>[4x]AHI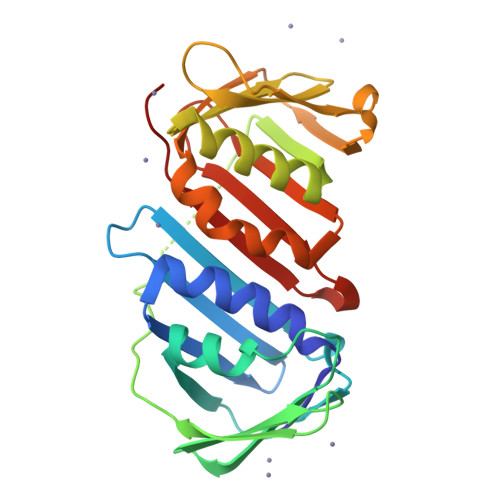VYDDVRDLKAIIQALLKLVDEALFDIKPEGIQLVAIDKAHISLIKIELPKEMFKEYDVPEEFKFGFNTQYMSKLLKAAKRKEEIIIDADSPEVVKLTLSGALNRVFNVNNIEVLPPEVPEVNLEFDIKATINASGLKNAIGEIAEVADTLLISGNEEKVVVKGEGENKVEVEFSKDTGSLADIEFNKESSSAYDVEYLNDIISLTKLSDYVKVAFADQKPMQLEFNMEGGGKVTYLLAPKLS> AS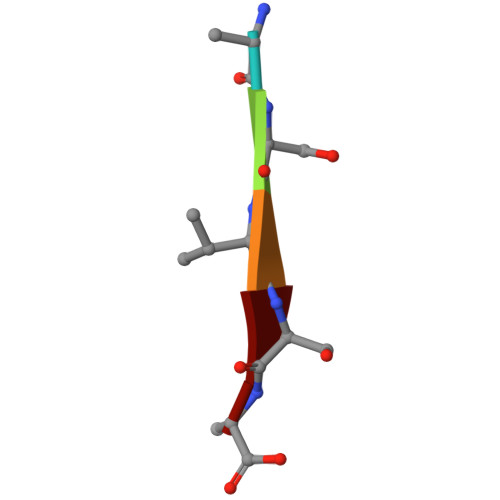VSA>NAADGIFFPALEQNMMGAVLINENDEVMFFNPAAEKLWGYKREEVIGNNIDMLIPRDLRPAHPEYIR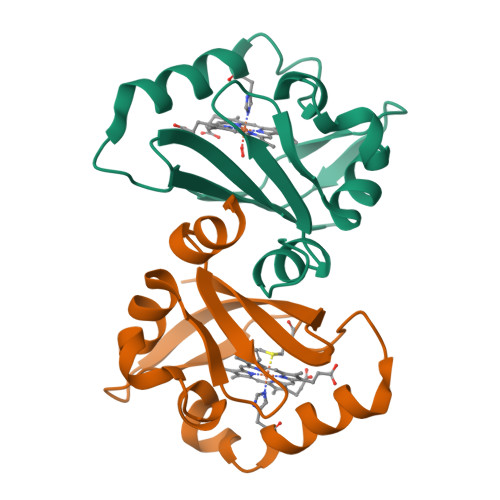HNREGGKARVEGMSRELQLEKKDGSKIWTRFALSKVSAEGKVYYLALVRDAS[2x]> E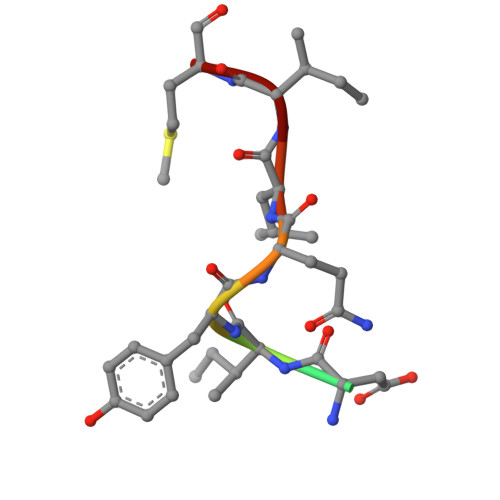DDIYQLIM>[6x]MSLQLLRNTRIFVSTVKTGHNKTNTQEILVQDDISWGQDSNSTDITVNEAGPRPTRGSKRFNDSLNAAEWSFSTYILPYKDKNTSKQIVPDYMLWHALSSGRAINLEGTTGAHNNATNFMVNFKDNSYHELAMLHIYILTDKTWSYIDSCQINQAEVNVDIEDIGRVTWSGNGNQLIPLDEQPFDPDQIGIDDETYMTIQGSYIKNKLTILKIKDMDTNKSYDIPITGGTFTINNNITYLTPNVMSRVTIPIGSFTGAFELTGSLTAYLNDKSLGSMELYKDLIKTLKVVNRFEIALVLGGEYDDERPAAILVAKQAHVNIPTIETDDVLGTSVEFKAIPSDLDAGDEGYLGFSSKYTRTTINNLIVNGDGATDAVTAITVKSAGNVTTLNRSATLQMSVEVTPSSARNKEVTWAITAGDAATINATGLLRADASKTGAVTVEATAKDGSGVKGTKVITVTAGG;>[3x]MFYSLMRESKIVIEYDGRGYHFDALSNYDASTSFQEFKTLRRTIHNRTNYADSIINAQDPSSISLAINFSTTLIESNFFDWMGFTREGNSLFLPRNTPNIEPIMFNMYIINHNNSCIYFENCYVSTVDFSLDKSIPILNVGIESGKFSEVSTFRDGYTITQGEVLPYSAPAVYTNSSPLPALISASMSFQQQCSWREDRNIFDINKIYTNKRAYVNEMNASATLAFYYVKRLVGDKFLNLDPETRTPLIIKNKYVSITFPLARISKRLNFSDLYQVEYDVIPTADSDPVEINFFGERK;>[12x]MSTENRVIDLVVDENVPYGLLMQFMDVDDSVYPSTSKPVDLTDFSLRGSIKSSLEDGAETVASFTTAIVDAAQGVASISLPVSAVTTIASKASKERDRYNPRQRLAGYYDVIITRTAVGSAASSFRIMEGKVYISDGVTQ;>MRLPDPYTNPEYPGLGFESVNLVDNDPMIRDELPNGKVKEVKISAQYWGINISYPELFPDEYAFLDSRLLEYKRTGDYLDVLLPQYEAFRVRGDTKSVTIPAGQKGSQIILNTNGTLTGQPKAGDLFKLSTHPKVYKITNFSSSGNVWNISLYPDLFITTTGSEKPVFNGILFRTKLMNGDSFGSTLNNNGTYSGISLSLRESL[6x];>[3x]MKKILDSAKNYLNTHDKLKTACLIALELPSSSGSAATYIYLTDYFRDVTYNGILYRSGKVKSISSHKQNRQLSIGSLSFTITGTAEDEVLKLVQNGVSFLDRGITIHQAIINEEGNILPVDPDTDGPLLFFRGRITGGGIKDNVNTSGIGTSVITWNCSNQFYDFDRVNGRYTDDASHRGLEVVNGTLQPSNGAKRPEYQEDYGFFHSNKSTTILAKYQVKEERYKLQSKKKLFGLSRSYSLKKYYETVTKEVDL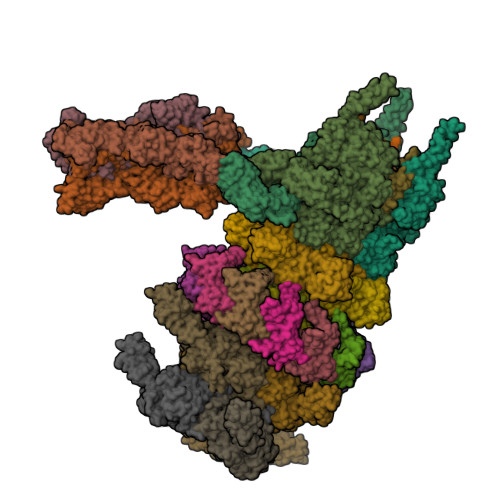DFNLAAKFIPVVYGVQKIPGIPIFADTELNNPNIVYVVYAFAEGEIDGFLDFYIGDSPMICFDETDSDTRTCFGRKKIVGDTMHRLAAGTSTSQPSVHGQEYKYNDGNGDIRIWTFHGKPDQTAAQVLVDIAKKKGFYLQNQNGNGPEYWDSRYKLLDTAYAIVRFTINENRTEIPEISAEVQGKKVKVYNSDGTIKADKTSLNGIWQLMDYLTSDRYGADITLDQFPLQKVISEAKILDIIDESYQTSWQPYWRYVGWNDPLSENRQIVQLNTILDTSESVFKNVQGILESFGGAINNLSGEYRITVEKYSTNPLRINFLDTYGDLDLSDTTGRNKFNSVQASLVDPALSWKTNSITFYNSKFKEQDKGLDKKLQLSFANITNYYTARSYADRELKKSRYSRTLSFSVPYKFIGIEPNDPIAFTYERYGWKDKFFLVDEVENTRDGKINLVLQEYGEDVFINSEQVDNSGNDIPDISNNVLPPRDFKYTPTPGGVVGAIGKNGELSWLPSLTNNVVYYSIAHSGHVNPYIVQQLENNPNERMIQEIIGEPAGLAIFELRAVDINGRRSSPVTLSVDLNSAKNLSVVSNFRVVNTASGDVTEFVGPDVKLAWDKIPEEEIIPEIYYTLEIYDSQDRMLRSVRIEDVYTYDYLLTYNKADFALLNSGALGINRKLRFRIRAEGENGEQSVGWATI;>MISNNAPAKMVLNSVLTGYTLAYIQHSIYSDYDVIGRSFWLKEGSNVTRRDFTGIDTFSVTINNLKPTTTYEVQGAFYDSIIDSELLNAQIGINLSDKQTFKMKSAPRITGARCESEPVDVGVGAPIVYIDTTGEADYCTIELKDNSNANNPWVKYYVGALMPTIMFGGVPIGSYKVRISGQISLPDGVTIDSSGYYEYPNVFEVRYNFVPPAAPINIVFKAARIADGKERYDLRVQWDWNRGAGANVREFVLSYIDSAEFVRTGWTKAQKINVGAAQSATIISFPWKVEHKFKVSSIAWGPDAQDVTDSAVQTFILNESTPLDNSFVNETGIEVNYAYIKGKIKDGSTWKQTFLIDAATGAINIGLLDAEGKAPISFDPVKKIVNVDGSVITKTINAANFVMTNLTGQDNPAIYTQGKTWGDTKSGIWMGMDNVTAKPKLDIGNATQYIRYDGNILRISSEVVIGTPNGDIDIQTGIQGKQTVFIYIIGTSLPAKPTSPAYPPSGWSKTPPNRTSNTQNIYCSTGTLDPVTNQLVSGTSWSDVVQWSGTEGVDGRPGATGQRGPGMYSLAIANLTAWNDSQANSFFTSNFGSGPVKYDVLTEYKSGAPGTAFTRQWNGSAWTSPAMVLHGDMIVNGTVTASKIVANNAFLSQIGVNIIYDRAAALSSNPEGSYKMKIDLQNGYIHIR[3x];>MTDKLIRELLIDVKQKGATRTAKSIENVSDALENAAAASELTNEQLGKMPRTLYSIERAADRAAKSLTKMQASRGMAGITKSIDGIGDKLDYLAIQLIEVTDKLEIGFDGVSRSVKAMGNDVAAATEKVQDRLYDTNRALGGTSKGFNDTAGAAGRASRALGNTSGSARGATRDFAAMAKIGGRLPIMYAALASNVFVLQTAFESLKVGDQLNRLEQFGTIVGTMTGTPVQTLALSLQNATNGAISFEEAMRQASSASAYGFDSEQLEQFGLVARRAAAVLGVDMTDALNRVIKGVSKQEIELLDELGVTIRLNDAYENYVKQLNATSTGIKYTVDSLTTYQKQQAYANEVIAESTRRFGYLDDALKATSWEQFAANANSALRSLQQSAATYLNPVMDTLNTFLYQTKSSQMRVSAMARSASAKTTPAENVTALIENAVGAREDLDTYLKESEERVKKAQELKQQLDDLKAKQAATAPIANALTAGGIGGDESNKLVVQLTNELARQNKEIEERTKTEKVLRQAVQDTGEALLRNGKLAEQLGAKMKYADTAVPGDKGVFEVDPNNLKAVSEIQKNFDFLKKSSSDTANNIRMAASSITNAKKASSDLNSVVKAVEDTSKVTGQSADTLVKNLNLGFSSLDQMKAAQKGLSEYVTAMDKSEQNALEVAKRKDEVYNQTKDKAKAEAAAREVLLRQQQEQLTAAKALLAINPNDPEALKQVAKIETEILNTKAQGFENAKKTKDYTDKILGVDREIALLNDRTMTSTQYRLAQLRLELQLEQEKTELYSKQADGQAKVEQSRRAQAQISREIWEAEKQGTASHVSALMDALEVSQTQRNVTGQSQILTERLSILQQQLELSKGNTEEELKYRNEIYKTSAALEQLKKQRESQMQQQVGSSVGATYTSTTGLIGEDKDFADMQNRMASYDQAISKLSELNSEATAVAQSMGNLTNAMIQFSQGSLDTTSMIASGMQTVASMIQYSTSQQVSAIDQAIAAEQKRDGKSEASKAKLKKLEAEKLKIQQDAAKKQIIIQTAVAVMQAATAVPYPFSIPLMVAAGLAGALALAQASSASGMSSIADSGADTTQYLTLGERQKNVDVSMQASSGELSYLRGDKGIGNANSFVPRAEGGMMYPGVSYQMGEHGTEVVTPMVPMKATPNDQLSDGSKTTSGRPIILNISTMDAASFRDFASNNSTAFRDAVELALNENGTTLKSLGNS[3x]>MRIPLVGKDSIESKDIGFTLIHEHLRVFSEAVRQQWPHLYNEDEEFRNAVNEVKRAMQFGVKTIVDPTVMGIGRDIRFMEKVVKATGINLVAGTGIYIFIDLPFYFLNRSIDEIADLFIHDLKEGIQGTLNKAGFVKIAADEPGITKDVEKVIRAAAIANKETKVPIITHSNAHNNTGLEQQRILTEEGVDPG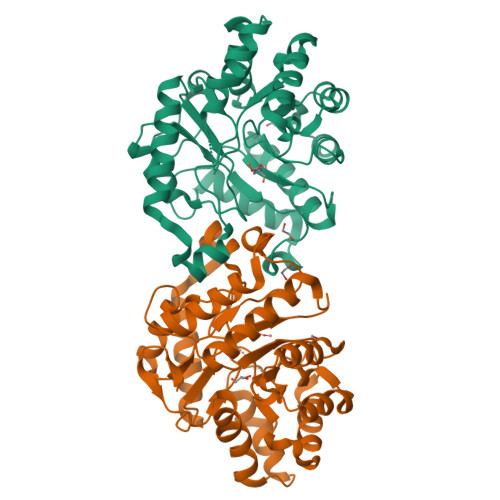KILIGHLGDTDNIDYIKKIADKGSFIGLDRYGLDMSLPVDKRNETTLRLIKDGYSDKIMISHDYCCTIDLGTAKPEYKPKLAPRWSITLIFEDTIPFLKRNGVNEEVIATIFKENPKKFFS[4x]> YRLEVGIQAMEHLIHVLQTDRSDSEIIGYALDTLYNIISNEEEEEVEENSTRQSEDLGSQFTEIFIKQQENVTLLLSLLEEFDFHVRWPGVKLLTSLLKQLGPQVQQIILVSPMGVSRLMDLLADSREVIRNDGVLLLQALTRSNGAIQKIVAFENAFERLLDIISEEGNSDGGIVVEDCLILLQNLLKNNNSNQNFFKEGSYIQRMKPWFEVGDENSGWSAQKVTNLHLMLQLVRVLVSPTNPPGATSSCQKAMFQCGLLQQLCTILMATGVPADILTETINTVSEVIRGCQVNQDYFASVNAPSNPPRPAIVVLLMSMVNERQPFVLRCAVLYCFQCFLYKNQKGQGEIVSTLLPSTIDATGNSVSAGQLLCGGLFSTDSLSNWCAAVALAHALQENATQKEQLLRVQLATSIGNPPVSLLQQCTNILSQGSKIQTRVGLLMLLCTWLSNCPIAVTHFLHNSANVPFLTGQIAENLGEEEQLVQGLCALLLGISIYFNDNSLESYMKEKLKQLIEKRIGKENFIEKLGFISKHELYSRASQKPQPNFPSPEYMIFDHEFTKLVKELEGVITKAIY

The golgin p115, which forms stable homodimers, is recruited to membranes in a nucleotide-dependent manner by the guanosine triphosphatase (GTPase) Rab1a and belongs to the family of tethers containing an extended coiled-coil region. p115 is among the best characterized representatives of long coiled-coil tethers. The architecture of p115 comprises a long central coiled-coil region, a large globular N-terminal domain and a C-terminal acidic region. p115 binds to a specific set of soluble N-ethylmaleimide-sensitive-factor attachment protein receptors (SNAREs), aiding formation of a cis-SNARE complex that promotes the antero-grade ER-to-Golgi transport by targeting COP II vesicles to the Golgi apparatus. In addition to its major role in exocytotic transport, p115 functions in retrograde Golgi-to-ER trans-port, intra-Golgi transport and Golgi biogenesis of the Golgi apparatus, due to essential interactions with the coat-protein complex I (COP I) subunit β-COP and the conserved-oligomeric-Golgi complex (COG) subunit COG2.

We used a construct comprising the globular head region of p115 (p115GHR, residues Asp54 to Tyr629) for crystallization. The fragment lacks 53 N-terminal residues that are predicted to be disordered and the C-terminal coiled-coil domain (p115CC). p115GHR consists of a multi-helical β-catenin-like armadillo fold arranged in a regular right-handed superhelix. We observe 10 classical armadillo repeats (ARM1-ARM10) and one non-canonical repeat which we termed USO repeat, after the yeast homolog of p115, Uso1p. ARM1 and ARM2 are connected by a highly acidic and flexible loop (residues 92–110), which is not visible in the electron density. The armadillo repeats exhibit long loops (5 to 13 residues) in ARM5-ARM9. This structural motif of elongated loops culminates in the formation of a short helix inserted in the H2-H3 loop (37 residues) of the terminal USO repeat which we named the USO helix. It folds back into the superhelical groove, leading to a globular C-terminus of p115GHR and covering helices H3 of ARM8-ARM9, while the USO helix points into the center of the groove. In the crystal structure, a dimeric arrangement between p115GHR molecules results from their packing along a dyad axis. The USO helix and the USO repeat helix H2 are part of the dimer interface which covers only 635 Å2 (∼2.6%) of the total 24,000 Å2 of solvent-accessible surface (SAS).> AAAAAAAA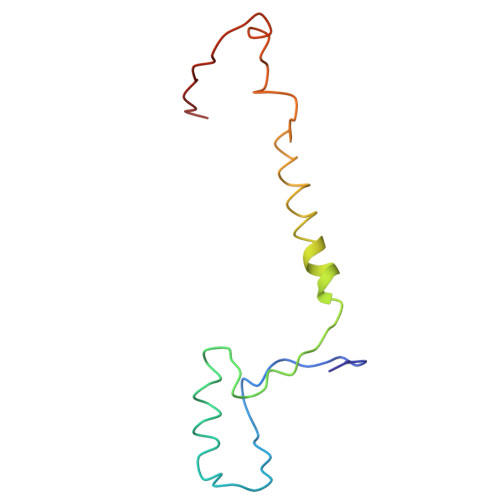AAAAAAAAAAAAAAAAAAAAAAAAAAAAAAAAAAAAAAAAAAAAAAAAAAAAAAAAAAAAAAAAAAAAAAAAAAAAAAAAAAAAAA> MWATLPLLCAGAWLLGVPVCGAAELCVNSLEKFHFKSWMSKHRKTYSTEEYHHRLQTFASNWRKINAHNNGNHTFKMALNQFSDMSFAEIKHKYLWSEPQNCSATKSNYLRGTGPYPPSVDWRKKGNFVSPVKNQGACGSSWTFSTTGALESAIAIATGKMLSLAEQQLVDCAQDFNNHGCQGGLPSQAFEYILYNKGIMGEDTYPYQGKDGYCKFQPGKAIGFVKDVANITIYDEEAMVEAVALYNPVSFAFEVTQDFMMYRTGIYSSTSCHKTPDKVNHAVLAVGYGEKNGIPYWIVKNSWGPQWGMNGYFLIERGKNMCGLAACASYPIPLV

Cathepsin H is a lysosomal cysteine protease of the papain superfamily involved in protein degradation. For preventing premature activation, cysteine proteases are synthesized as inactive proenzymes called zymogens that contain a prodomain and a mature (catalytic) domain, and the removal of the prodomain leads to the activation of the enzymes. Upon activation, cathepsin H displays a distinct proteolytic activity among the papain superfamily, functioning predominantly as an aminopeptidase that cleaves a single N-terminal residue from a polypeptide chain. Unique among papain-like cysteine proteases, the mini-chain (the octapeptide EPQNCSAT from the prodomain) remains bound to cathepsin H through a disulfide bond and is essential for the aminopeptidase activity.

We also mutated residue Cys26 in the active site to Ser to avoid potential autoprocessing and determined the crystal structure of procathepsin H C26S mutant at 1.66 Å resolution. The wild type and mutant structures are essentially identical with an RMSD of 0.14 Å for all Cα atoms. Ligand/ion in the structure of C26S mutant: N-acetyl-D-glucosamine, β-D-mannopyranose, α-D-mannopyranose, sulfate ion, chloride ion, trehalose. The helical subdomain is positioned on top of the right domain of the mature domain while the C-terminal extended portion traverses the substrate binding cleft toward the N-terminus of the mature domain, preventing access of the substrates to the active site. The mini-chain (Glu76P-Thr83P) in procathepsin H connects the N-terminal helical subdomain and the C-terminal linker in the prodomain, and is located right above the active site cleft of the mature domain. It is largely solvent-exposed and, except for the disulfide bond between Cys80P and Cys212, makes limited water mediated hydrogen bond interactions with the residues lining the cleft. However, these three catalytic residues in procathepsin H are shielded by a group of hydrophobic residues Tyr72P, Leu73P, Trp74P from the prodomain, which effectively blocks the access to the catalytic Cys and prevents external substrates from entering the binding site. Structural comparison with cathepsin H revealed that the mini-chain in procathepsin H runs in the direction opposite to that of the substrates while the mini-chain in cathepsin H follows the substrate binding direction, suggesting that the negatively charged C-terminal carboxyl group in the mini-chain of cathepsin H is positioned to interact with the N-terminal amino group of the substrate whereas the cleaved mini-chain in procathepsin H needs to reorient to be involved in such interaction. In addition to the proteolytic processing of the prodomain, the activation of procathepsin H requires the reorientation and repositioning of the mini-chain along the active site in the substrate-binding direction from the direction opposite to a bound substrate.Mevalonate kinase is central to the isoprenoid biosynthesis pathway. Mevalonate kinases (MK) catalyse the phosphorylation of mevalonate. Mevalonate kinases belong to the GHMP kinase superfamily, which includes enzymes such as galactokinase, homoserine kinase, MK and phosphomevalonate kinase. The His tag was not resolved in the structure. Like all GHMP superfamily enzymes, each monomer is composed of two domains: an N-terminal domain and a C-terminal domain separated by a cleft.

In this work, we have identified, purified and characterized, both biochemically and structurally, two previously uncharacterized mevalonate kinases originating from the extremotolerant tardigrade R. varieornatus (Hashimoto et al., 2016; MKvar) and the psychrophilic archaeon M. burtonii (MKbur; Allen et al., 2009). As part of this study, the crystal structure of MKvar with mevalonate in the active site was determined to 2 Å resolution and the crystal structure of MKbur was determined to 2.2 Å resolution. The structures of the archaeal MKs MKmaz and MKbur are highly similar and their sequence alignment shows 61.1% identity and an r.m.s.d. of 0.77 Å; however, their thermostability assay and DSF results show a striking 20°C difference. Measuring residual activity after incubation at temperatures ranging from 25 to 80°C for 5 min revealed that the T 50 values were 40°C for MKbur and 62°C for both MKvar and MKmaz. MKbur, as expected from its psychrophilic origin, appears to conserve activity at low temperature and has relatively low thermostability. In MKvar, Thr119 and Ile215 align with Thr104 and Ile196, respectively, in human MK. MKbur has a conserved Ile residue; however, Thr119, which can be found at the N-terminus of the α4 helix in MKvar, is not present in the N-terminal region of α1 in MKbur.

>[2x]MITCSAPGKVYLFGEHAVVYGEPAICCAVDIRTRVTVSPADTITISSSLGTTGIDFEVHPYVSAVLERFQDISSFDGVDLRISSDIPVGSGLGSSAAVTVATIKAMDTLLDLGLELDDIAKMGHEVEQNIQGTASPTDTYVCTMGGVVLIPQRKKLELIDCGILIGNTNIFSSTKELVGNVADLNERFPDVVGPVLSSIGKLSVIGEGLVNDRDYVSVGELMNIDQGLLDAIGVSCAELSSLIYAARESGAYGSKITGAGGGGCMVAISPRENVDSVAEAIGMAGGKVVVANATDIGVRVECQLVPRGSLEHHHHHH> MQSTPLLQIQPHFHVEVIEPKQVYLLGEQANHALTGQLYCQILPLLNGQYTLEQIVEKLDGEVPPEYIDYVLERLAEKGYLTEAAPELSSEVAAFWSELGIAPPVAAEALRQPVTLTPVGNISEVTVAALTTALRDIGISVQTPTEAGSPTALNVVLTDDYLQPELAKINKQALESQQTWLLVKPVGSVLWLGPVFVPGKTGCWDCLAHRLRGNREVEASVLRQKQAQQQRNGQSGSVIGCLPTARATLPSTLQTGLQFAATEIAKWIVKYHVNATAPGTVFFPTLDGKIITLNHSILDLKSHILIKRSQCPTCGDPKILQHRGFEPLK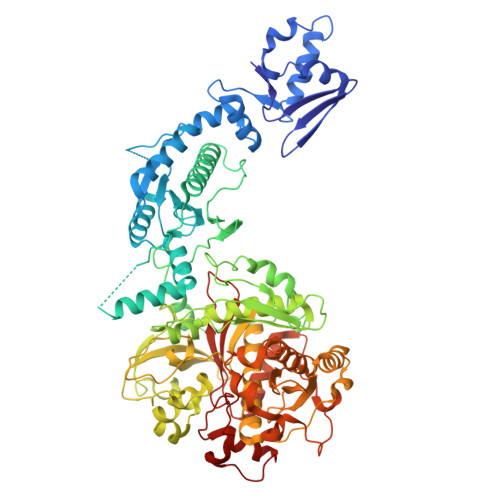LESRPKQFTSDGGHRGTTPEQTVQKYQHLISPVTGVVTELVRITDPANPLVHTYRAGHSFGSATSLRGLRNTLKHKSSGKGKTDSQSKASGLCEAVERYSGIFQGDEPRKRATLAELGDLAIHPEQCLCFSDGQYANRETLNEQATVAHDWIPQRFDASQAIEWTPVWSLTEQTHKYLPTALCYYHYPLPPEHRFARGDSNGNAAGNTLEEAILQGFMELVERDGVALWWYNRLRRPAVDLGSFNEPYFVQLQQFYRENDRDLWVLDLTADLGIPAFAGVSNRKTGSSERLILGFGAHLDPTIAILRAVTEVNQIGLELDKVPDENLKSDATDWLITEKLADHPYLLPDTTQPLKTAQDYPKRWSDDIYTDVMTCVNIAQQAGLETLVIDQTRPDIGLNVVKVTVPGMRHFWSRFGEGRLYDVPVKLGWLDEPLTEAQMNPTPMPF> MQRAGCGIVRPGRGCHTTPLYCSLATISTGVFDHLPFQHRRQHAFNTLPLHDANHFGGRTAYLREIGPVNIKKSGRRFKKDLRTVQFNVDIWCAQQTLRKRWKQRDWEVIEVPFRLAPAEQQRVIPE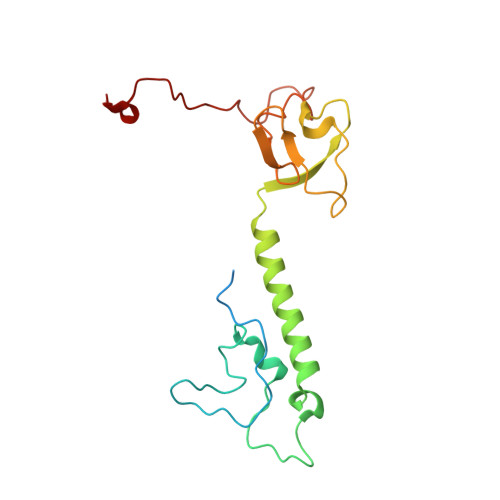MYTDVPPMTDPERHDFSNIRNKVYDREELQGVLFGASGPLPYPPLQRIDRQAMTLDKFL> MTDVDKRKIKIILNGEMEEAELHMITSPNRHCCLKIFHNNNQLAESNDTDYFSCFADLRNQLKNIIFLCKGAKINVYPSAMSRDMSDGIVAYETTLGQPGLPENQVHIFDFEDKYVDITPEEQRKFHSQWFESLVDHHHHHH;> MAGGIGNKGDYIITYRGDTRSFTEIFDKGFETLGPSKDLYKHALDNRAPPSDFVSTTIDPTKTISFATKYGQKSGYMYT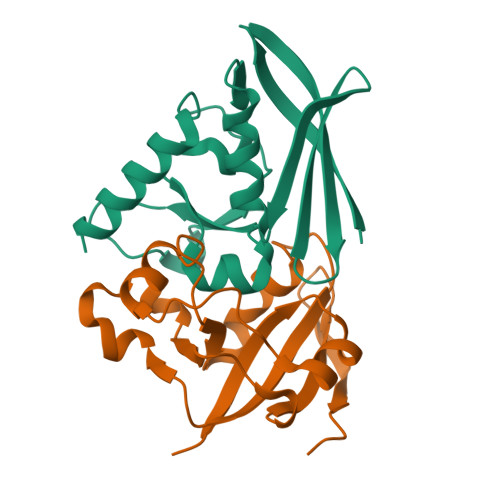MKTNHGIDVNKALGARSPFAAEAEIAMPGGVRAEDILGARAVNADGEMWDYTILNPKRYGK>MAVTDLRDVEEDVKGKLDEWLNALVHLDKQQVERIYEELQGEMKHVLDFEIINYYKLLYTRYLIMKRDISALEEELDKLKKVYKKYSPFQKLLYMYGRGLLCCLQYRWKDGLDYLLKTEVMAKEQGYHETGLYYNIALAYTHLDIHHLAIHFVNMALEGFRSEYKFRNIINCQILIAVSYTEKGQYEEALKMYESILREATSFADKDVLLAITLSNMGSIYYKKGKYQQAKKYYLDSLQLQKQIDLNYLDTIYEMALVCIKLEELEEARTL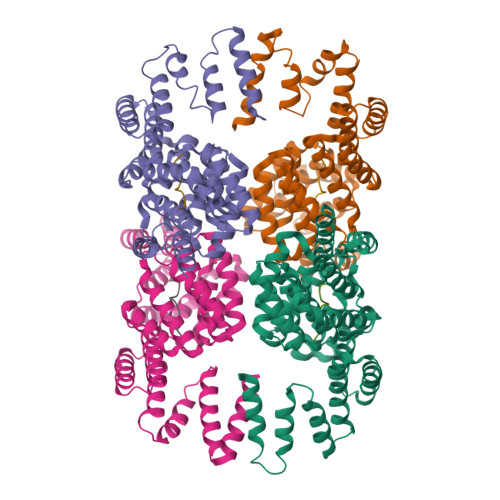IDKGIDAAKQEERFNAKLYLLLMLRYKYFEEAKDYKAFLENEAIPLYKSAGNKIELKKVYVELAEHFSSLSRFEESNRYYRLVIDLMNDNKEERSHHHHHH[12x];>SSKPDIVG[12x]N-(alpha-L-Fucopyranosyl)benzamide | C13 H17 N 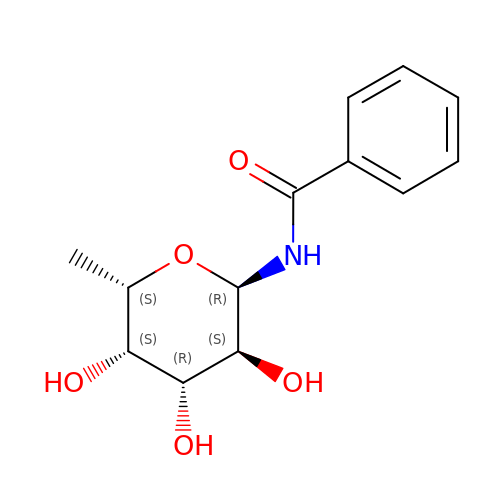O5 | ZYWNMRPOYLXAAW-HTUCIKCGSA-N> PEGLEQLEAQTNFTKRELQVLYRGFKNECPSGVVNEDTFKQIYAQFFPHGDASTYAHYLFNAFDTTQTGSVKFEDFVTALSILLRGTVHEKLRWTFNLYD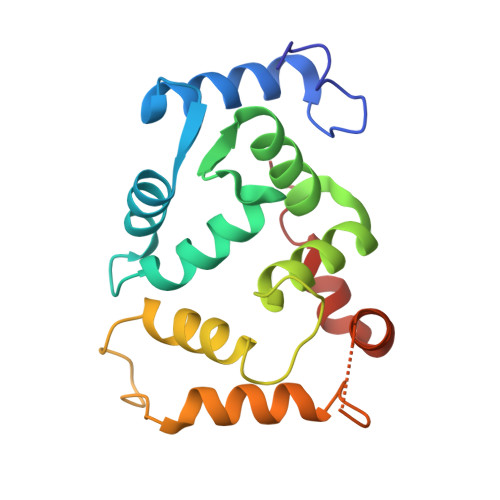INKDGYINKEEMMDIVKAIYDMMGKYTYPVLKEDTPRQHVDVFFQKMDKNKDGIVTLDEFLESCQEDDNIMRSLQLFQNVM> MLQQPTGGYTTLEQFAFTIRNDGTNATPTQFLQLLSYEATENELVKKTIPTPETH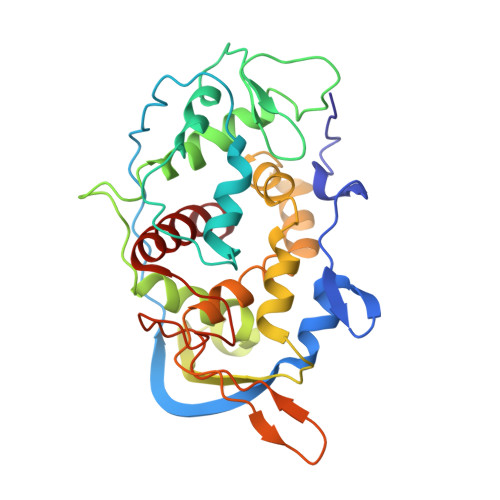LPSARNVPGNVYIEDAITQALFGISAQNVNAHGYFSRLSALALPNTSARLGLDGVIYNSETINIPFYDPAAVANFAATYAKLGNASTPRYRADMIDIYAHVGLELAGTDAERAAGVMPVKRAKFDSWEGSLISLSRDVVNWKILAFLIDLCSLEGEALRAFKTRNRDVFRMMLFIMSTAVAANVVNRKVTKRVDRVLEYIGVNSMRTAGRTATITYDLSRHEFAAKFLQLTFTRWN> ADYDLKFGMNAGTSSNEYKAAEMFAKEVKEKSQGKIEISLYPSSQLGDDRAMLKQLKDGSLDFTFAESARFQLFYPEAAVFALPYVISNYNVAQKALFDTEFGKDLIKKMDKDLGVTLLSQAYNGTRQTTSNRAINSIADMKGLKLRVPNAATNLAYAKYVGASPTPMAFSEVYLALQTNAVDGQENPLAAVQAQKFYEVQKFLAMTNHILNDQLYLVSNETYKELPEDLQKVVKDAAENAAKYHTKLFVDGEKDLVTFFEKQGVKITHPDLVPFKESMKPYYAEFVKQTGQKGESALKQIEAINPHHHHHH

Tripartite ATP-independent periplasmic (TRAP) transporters are secondary transporters that have evolved an obligate dependence on a substrate-binding protein (SBP) to confer unidirectional transport. We investigated the significance of this interaction using the sialic acid-specific SBP, SiaP, from the Haemophilus influenzae virulence-related SiaPQM TRAP transporter. The first structure of a TRAP SBP revealed that the charge of the carboxylate group of the ligand, sialic acid, was neutralized by an arginine residue, Arg-147, in SiaP, which sequence analysis had revealed to be the most highly conserved residue, being present in 98% of TRAP SBPs of the common DctP family. Using in vitro, in vivo, and structural methods applied to SiaP, we demonstrate that the coordination of the acidic ligand moiety of sialic acid by the conserved arginine (Arg-147) is essential for the function of the transporter as a high affinity scavenging system.

We attempted to crystallize the wild-type protein with this non-cognate sialylamide ligand and were able to collect data to atomic resolution of 1.05 Å where ab initio phasing was applied to remove any model bias. Strikingly, the ligand appeared to be coordinated exactly as Neu5Ac, including the positioning of all waters in the binding pocket, and careful refinement of the structure revealed that the bound species was in fact Neu5Ac, based on analysis of H-bonding patterns (interaction with waters), B-factors of the carboxylate, and also considering expected bond lengths for unrestrained refinement of oxygen and nitrogen atoms. Mass spectrometry data confirmed the presence of trace amounts of Neu5Ac in the sialylamide sample despite purification after synthesis using silica and ion-exchange chromatography and checked by one-dimensional 1H NMR. The finding that the wild-type protein was able to selectively bind this minor contaminating component, while R147E protein exposed to the same stock crystallized with the bound sialylamide, confirms the important role of the Arg-147 residue in the selectivity of SiaP for its cognate ligand. Crystallization of the wild-type SiaP with the same preparation of sialylamide revealed that the arginine is able to “fish out” even the minimal amounts of Neu5Ac present in this sialylamide preparation, analogous to conditions of limited environmental nutrients. These data also suggest that sialylamide probably is not a true ligand for wild-type SiaP, and binding detected in Muller et al. was likely due to this low level of contamination with Neu5Ac. Binding of N-acetylneuraminic acid (Neu5Ac) to C-terminally hexahistidine-tagged wild-type SiaP-His6 yielded a KD of 0.14 ± 0.04 μm, in close agreement with published data for native or N-terminally His-tagged versions.>[2x]MVAAQKKKAQDEYGAASITILEGLEAVRKRPGMYIGSTGERGLHHLIWEVVDNAVDEAMAGYATTVNVVLLEDGGVEVADDGRGIPVATHASGIPTVDVVMTQLHAGGKFDSDAYAISGGLHGVGVSVVNA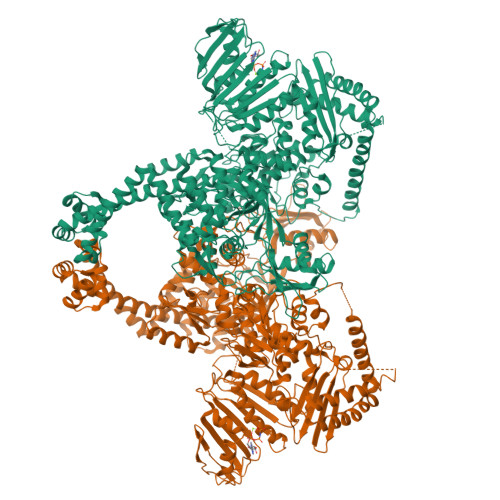LSTRLEVEIKRDGYEWSQVYEKSEPLGLKQGAPTKKTGSTVRFWADPAVFETTEYDFETVARRLQEMAFLNKGLTINLTDERVTQDEVVDEVVSDVAEAPKSASERAAESTAPHKVKSRTFHYPGGLVDFVKHINRTKNAIHSSIVDFSGKGTGHEVEIAMQWNAGYSESVHTFANTINTHEGGTHEEGFRSALTSVVNKYAKDRKLLKDKDPNLTGDDIREGLAAVISVKVSEPQFEGQTKTKLGNTEVKSFVQKVCNEQLTHWFEANPTDAKVVVNKAVSSAQARIAARKARELVRRKSATDIGGLPGKLADCRSTDPRKSELYVVEGDSAGGSAKSGRDSMFQAILPLRGKIINVEKARIDRVLKNTEVQAIITALGTGIHDEFDIGKLRYHKIVLMADADVDGQHISTLLLTLLFRFMRPLIENGHVFLAQPPLYKLKWQRSDPEFAYSDRERDGLLEAGLKAGKKINKEDGIQRYKGLGEMDAKELWETTMDPSVRVLRQVTLDDAAAADELFSILMGEDVDARRSFITRNAKDVRFLDVGDLTDTTLPPDDSLDRIEPVDIEQEMQRSYIDYAMSVIVGRALPEVRDGLKPVHRRVLYAMFDSGFRPDRSHAKSARSVAETMGNYHPHGDASIYDSLVRMAQPWSLRYPLVDGQGNFGSPGNDPPAAMRYTEARLTPLAMEMLREIDEETVDFIPNYDGRVQEPTVLPSRFPNLLANGSGGIAVGMATNIPPHNLRELADAVFWALENHDADEEETLAAVMGRVKGPDFPTAGLIVGSQGTADAYKTGRGSIRMRGVVEVEEDSRGRTSLVITELPYQVNHDNFITSIAEQVRDGKLAGISNIEDQSSDRVGLRIVIEIKRDAVAKVVINNLYKHTQLQTSFGANMLAIVDGVPRTLRLDQLIRYYVDHQLDVIVRRTTYRLRKANERAHILRGLVKALDALDEVIALIRASETVDIARAGLIELLDIDEIQAQAILDMQLRRLAALERQRIIDDLAKIEAEIADLEDILAKPERQRGIVRDELAEIVDRHGDDRRTRIIAA> SPAAQVDLRTLGYSQQQQEKIKPKVRS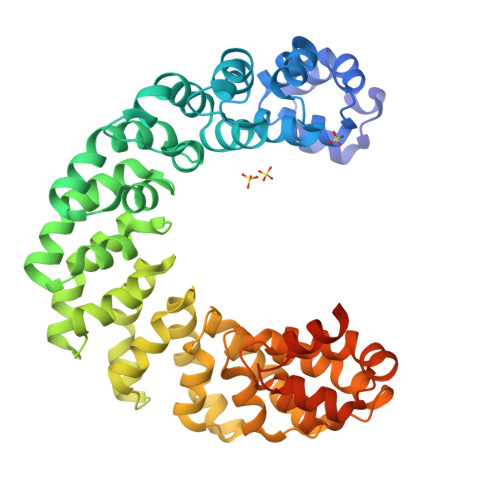TVAQHHEALVGHGFTHAHIVALSQHPAALGTVAVKYQDMIAALPEATHEAIVGVGKQWSGACALEALLTVAGELRGPPLQLDTGQLLKIAKRGGVTAVEVHHTWRNALTGAPLNLTPDQVVAIASNIGGKQALETVQRLLPVLCQDHGLTPQQVVAIASNGGGKQALETVQRLLPVLCQAHGLTPDQVVAIASHDGGKQALETVQRLLPVLCQDHGLTPQQVVAIASNIGGKQALETVQRLLPVLCQDHGLTPDQVVAIASNDGGKQALETVQRLLPVLCQDHGLTPEQVVAIASNGGGKQALETVQRLLPVLCQAHGLTPDQVVAIASHDGGKQALETVQRLLPVLCQDHGLTPAQAVAIANNNGGKQALETVQRLLPVLCQDHGLTPDQVVAIASNGGGKQALESIVAQLSCPDPALAALTNDHLVALACLGGR N-(6-AMINOHEXYL)HEXANE-1,6-DIAMINE | C12 H29 N3 | 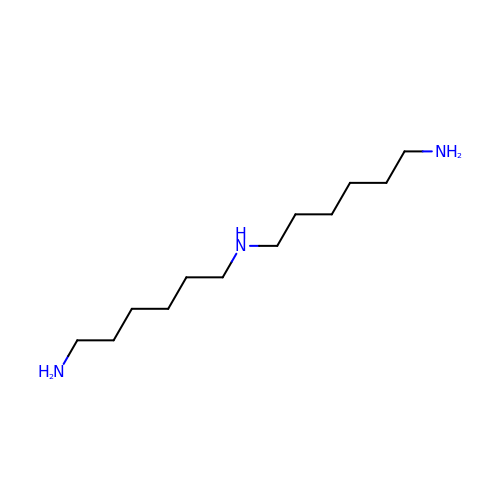MRNZSTMRDWRNNR-UHFFFAOYSA-N> HMKTVLMVAEKPSLAQSIAKILSRGSLSSHKGLNGACSVHEYTGTFAGQPVRFKMTSVCGHVMTLDFLGKYNKWDKVDPAELFSQAPTEKKEANPKLNMVKFLQVEGRGCDYIVLWLDCDKEGENICFEVLDAVLPVMNKAHGGEKTVFRARFSSITDTDICNAMACLGEPDHNEALSVDARQELDLRIGCAFTRFQTKYFQGKYGDLDSSLISFGPCQTPTLGFCVERHDKIQSFKPETYWVLQAKVNTDKDRSLLLDWDRVRVFDREIAQMFLN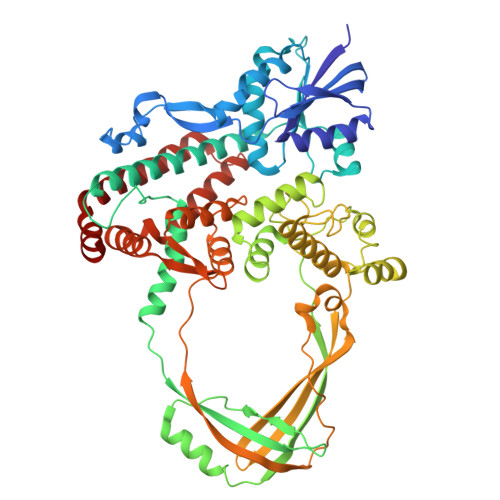MTKLEKEAQVEATSRKEKAKQRPLALNTVEMLRVASSSLGMGPQHAMQTAERLYTQGYISYPRTETTHYPENFDLKGSLRQQANHPYWADTVKRLLAEGINRPRKGHDAGDHPPITPMKSATEAELGGDAWRLYEYITRHFIATVSHDCKYLQSTISFRIGPELFTCSGKTVLSPGFTEVMPWQSVPLEESLPTCQRGDAFPVGEVKMLEKQTNPPDYLTEAELITLMEKHGIGTDASIPVHINNICQRNYVTVESGRRLKPTNLGIVLVHGYYKIDAELVLPTIRSAVEKQLNLIAQGKADYRQVLGHTLDVFKRKFHYFVDSIAGMDELMEVSFS3-fluoro-N'-[(E)-{5-[(pyrimidin-2-yl)sulfanyl]furan-2-yl}methylidene]benzohydrazide | C16 H11 F N4 O2 S | 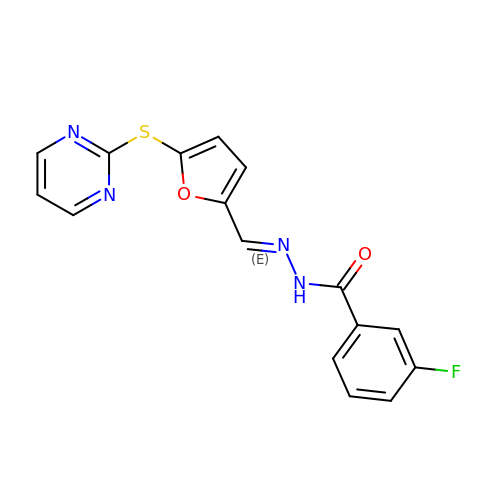DRXIKWHRYGIZNG-KEBDBYFISA-N> MVSVPRGQGGAAPAVVGQVSESARQAEAARQAWLQAHPAWSFQGRVAISKGRDGGSGRLDWQQDGPRYHVQLSAPVTRQSWVLTGDTTTGAGRLEGLDGGPRAGADAEQVLLEATGWTIPVNQMPDWVRALRIADAGAARVDLDEHGRPRTVQ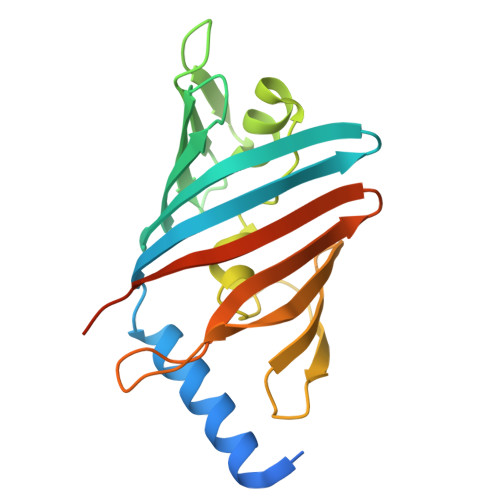QDGWTIDFLEWTPASAAQPELPRRIEARNGDAKVRLLVDQWTLSPAENLYFQSHHHHHH>[2x]TGVTENTICKYGYLIQMSNHYECKCIEGYVLINEDTCGKKVVCDKVENSFKACDEYAYCFDLGNKNNEKQIKCMCRTEYTLTAGVCVPNVCRDKVCGKGKCIVDPANSLTHTCSCNIGTILNQNKLCDIQGDTPCSLKCAENEVCTLEGNYYTCKEDPSSNGGGNTVDQADTSYSGTKHHHHHH

Pfs28 is a Plasmodium falciparum malaria transmission-blocking vaccine candidate that is anchored to the parasite surface through a C-terminal glycosylphosphatidylinositol (GPI) moiety, and plays a role in parasite survival in the mosquito midgut. Pfs28 contains epidermal growth factor (EGF)-like domains and is part of a family of sexual stage malaria proteins that includes the related vaccine antigen Pfs25. Pfs28 is a glycosylphosphatidylinositol-anchored protein expressed on the surface of zygotes and ookinetes and plays a similar role as Pfs25 in ookinete survival and traversal through the midgut. Pfs28 is a GPI-anchored protein, consisting of an N-terminal signal sequence, four EGF-like domains, and a C-terminal hydrophobic sequence that is the site of GPI attachment.

The construct used for crystallography consisted of V1-S173, comprising only the four EGF-like domains. The crystal structure of Pfs28 was solved to a resolution of 2.3 Å. The Pfs28 structure is comprised of four EGF-like domains in a triangular arrangement, with sides of 40 Å and 50 Å and a thickness of ~ 20 Å, with the overall structure stabilized by 10 disulfide bridges. EGF domains 1–3 adopt the characteristic structure, consisting of a major two-stranded β-sheet followed by a loop and a shorter two-stranded β-sheet, while only a single two-stranded β-sheet in EGF4 was observed. EGF domains 1 and 4 each have two disulfide bridges, while EGF domains 2 and 3 contain three disulfide bridges. Due to flexibility and a lack of clear density at the C-terminus of the protein, the C-terminal portion of EGF4 (residues S157-S173) could not be modelled. The major difference between the structures of the two antigens lies in the lack of the third disulfide bridge in EGF4 of Pfs28. This is reflected in the greater degree of disorder present in EGF4 of Pfs28 compared to Pfs25, such that its C-terminal region could not be resolved in the crystal structure. The residues shown to stabilize the triangular arrangement of the EGF domains in Pfs25 are conserved in Pfs28: Q14, M15, S16, H18, E20, K98, S112, C113, T131 and L135. However, the crystal packing of Pfs28 did not adopt a similar tile-like pattern and we also saw no evidence of interaction between Pfs25 and Pfs28 as measured by BLI.>AGLNTAAKAKGLKYFGSATDNPELTDSAYVAQLSNTDDFGQITPGNSMKWDATEPSQNSFSFANGDAVVNLANKNGQLMRCHTLVWHSQLPNWVSSGSWTNATLLAAMKNHITNVVTHYKGKCYAWDVVNEALNEDGTFRNSVFYQIIGPAYIPIAFATAAAADPDVKLYYNDYNIEYSGAKATAAQNIVKMIKAYGAK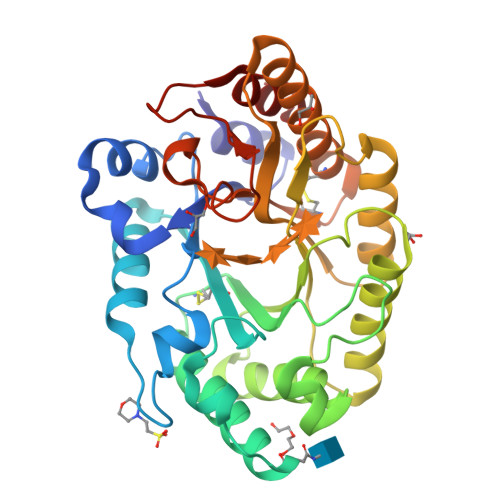IDGVGLQAHFIVGSTPSQSDLTTVLKGYTALGVEVAYTELDIRMQLPSTAAKLAQQSTDFQGVAAACVSTTGCVGVTIWDWTDKYSWVPSVFQGYGAPLPWDENYVKKPAYDGLMAGLGA[2x]> DYKDDDDLEVLFQGPGGSSAPARPNWLAYDWGLVFLVAAIVALGFVNLGSAAPDPVLLYRQSVALGLGLLLAFLLQFLSRRRLFGLAYPLYGASLLLLALVLVVGREINGARAWFVLGPLQFQPLELAKLGLLLALAKALEGRPIARVWDYALPALLTLPVVGLLLLQPDLGGALVVLFGVFVVVFVRGLPWRHLLVGLFALALLVPTAVWPNLKPYQRERVLIVLDPYRDPLGQGFQVIQSTIAIGSGGLFGKGYGQGTQAQLGFIPFRHTDFVFSVWAEEWGFVGVVGLLGLYGLLLARLFALALACPRLSDRLFLSGFAGMLGFQVVVNLGVALGVMPVTGLTLPLFSYGGSSLIATLAGLGLVLLVHRDRYQD;> MGTGRIHALALFFALALFLLGLRAWQLQVLEYERYALRSQGNYLKTEDIPAPRGKILDRKGRVLAQDRLVVDLVYTGGEVAFKERLLPLLGLEDLPQVTEPTVLKAGVPEALRPTLEELTAGQKNLYLRERIERYYPNPISGPVMGYVLRANAAQVKQGYSPEEEVGQAGLEAALEPYLRGKRGVRAVEVNVRGERLRETVLEEPTPGQDVVLTLDLALQRAAEKALEEALADINAGRRLNGLPEEKQVKGAIVALDPTTGEVLAMASAPSFDPNLFAKRPVPEEAKALLEDKNLPLLNRAVQPYTPGSTFKLATSYALLEEGYVTPATTYRCSPYIVFGGQVRRNWASRDMGPMTVREAIAWSCNTWYYQAVAQDPLGFVDRLARRARLLGLGEATGLEVAEKTGLLPTRAWK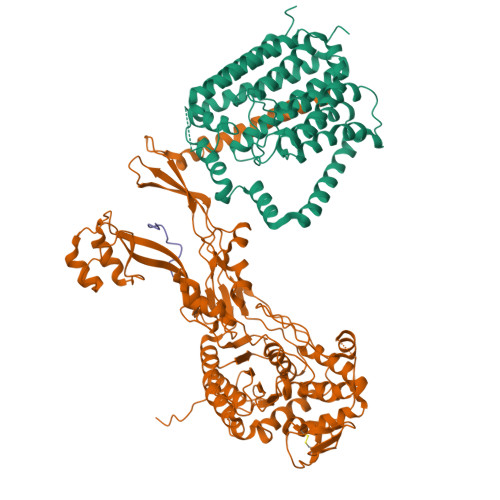REALGEPWYPGETLSVAIGQGAVLATPAQIARMLATIATGGNKPALHLVKAIGGVPVQPRWEKVPGRYWKVLQEGLRKTVSEGTARFVLGEFPVPTGGKTGTAETPGKRRGLEHAWYMGYGPTDGSPYPPLVVVAFFENGGEGSRVALPAVRKVMAAYWGIKGSLEVLFQGPEDQVDPRLIDGK>MDSLLNEKKKFIRHVLSNAPPGKVFDLISNLKTIFGSNAIIQNFIEDIISKYNEDNYILIPFESDEYIIICKESKSGNLYLHPNLKILANVNHLKRKVIDTTPLTKLDHPDILEKYRVACNNKLKEYVDIYYKKWSDHQTGNYPTVNIGSKHGLNVKCASSVYASECENKYNLFLLIC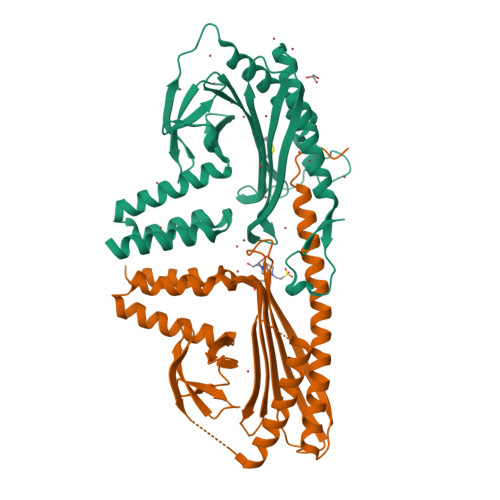CDRYYLKNFHASSWRSSWNVNFLEADQEIILTGTIDVVLTYFEDANINFKTRKVFEKRVSVTNDIENFASSILSVIRECENDVLYDLNHLIANTSSDLIKNTRKIIPLNAHHHHHH[2x]> XYVWLTDT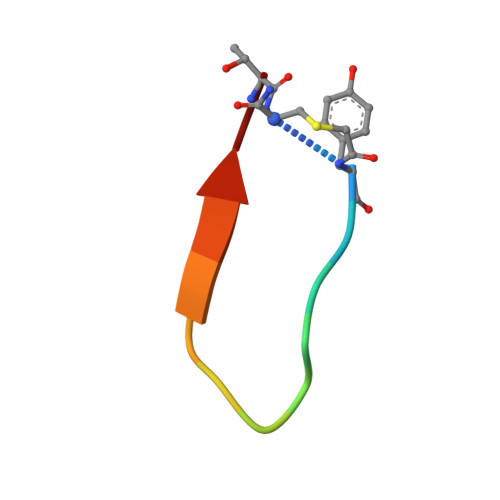WVLSRT>MGQEKLLFDQKYKIIKGEKKEKKKNQRANRREHQQKREIMRFKKSFTCIDMHTEGEAARIVTSGLPHIPGSNMAEKKAYLQENMDYLRRGIMLEPRGHDDMFGAFLFDPIEEGADLGIVFMDTGGYLNMCGHNSIAAVTAAVETGIVSVPAKATNVPVVLDTPAGLVRGTAHLQSGTESEVSNASIINVPSFLYQQDVVVVLPKPYGEVRVDIAFGGNFFAIVPAEQLGIDISVQNLSRLQEAGELLRTEINRSVKVQHPQLPHINTVDCVEIYGPPTNPEANYKNVVIFGNRQADRSPCGTGTSAKMATLYAKGQLRIGETFVYESILGSLFQGRVLGEERIPGVKVPVTKDAEEGMLVVTAEITGKAFIMGFNTML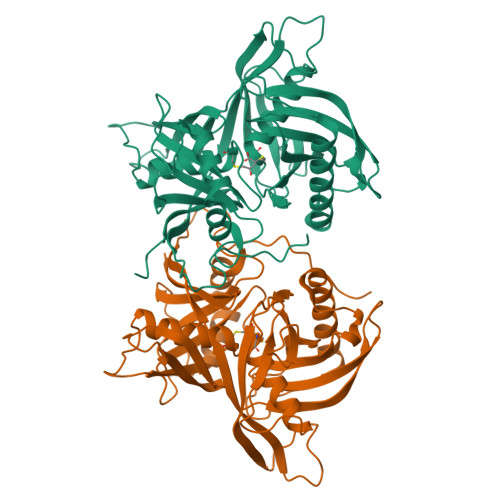FDPTDPFKNGFTLKQYIWSSSVDKLAAALEHHHHHH[2x]The Microrchidia (MORC) family of chromatin-remodelling ATPases is pivotal in forming higher-order chromatin structures that suppress transcription. All MORCs share three features: an N-terminal gyrase, heat shock protein 90, histidine kinase and MutL (GHKL) ATPase domain, a central CW-type zinc finger (CW) domain, and a divergent C-terminal domain (CTD) with predicted coiled coils (CCs). MORC2 possesses multiple DNA-binding sites that undergo structural rearrangement upon DNA binding. Importantly, MORC2 mediates chromatin remodelling via ATP hydrolysis-dependent DNA compaction in vitro, regulated by the phosphorylation state of its CTD.

As a MORC2 neuropathic mutant S87L was shown to have residual ATP hydrolysis activity, we have identified and utilised ATP hydrolysis mutant S87A. We determined a 2.4 Å cryo-electron microscopy (cryoEM) structure of full-length MORC2 ATPase-dead mutant (MORC2S87A) in the presence of AMP-PNP. The AMP-PNP density was visible in the cryoEM map and at the same location as found in the crystal structures. The presence of AMP-PNP density near the ATP lid in MORC2S87A model, confirmed that this mutant can bind but not hydrolyse ATP, mimicking S87L variant where some residual ATPase activity is still detected. S87A mutant had similar DNA binding affinity as wild-type MORC2, indicating that ATP binding did not affect MORC2 DNA binding. The dimerised ATPase domain is well-resolved in all the cryoEM maps, but no density is seen for CTD to model in the full-length MORC2PD, MORC2PD-DNA and MORC2S87A maps. The lag time for DNA compaction by MORC2S87A was 3.5 times longer than that of MORC2WT, with an eightfold increase in compaction time. We found that MORC2WT compacted DNA into a large DNA cluster, whereas MORC2S87A, MORC2N39A, MORC21-603 and MORC2604-1032 variants did not. Our investigation of the MORC2 S87A mutant based on the patient variant S87L, which retains ATP binding but has significantly lower ATPase activity, showed significantly slower DNA compaction than MORC2WT.

>[2x]MAFTNYSSLNRAQLTFEYLHTNSTTHEFLFGALAELVDNARDADATRIDIYAERREDLRGGFMLCFLDDGAGMDPSDAASVIQFGKAAKRTPESTQIGQYGNGLKSGSMRIGKDFILFTKKEDTMTCLFLSRTFHEEEGIDEVIVPLPTWNARTREPVTDNVEKFAIETELIYKYSPFRTEEEVMTQFMKIPGDSGTLVIIFNLKLMDNGEPELDIISNPRDIQMAETSPEGTKPERRSFRAYAAVLYIDPRMRIFIHGHKVQTKRLSCCLYKPRMYKYTSSRFKTRAEQEVKKAEHVARIAEEKAREAESKARTLEVRLGGDLTRDSRVMLRQVQNRAITLRREADVKKRIKEAKQRALKEPKELNFVFGVNIEHRDLDGMFIYNCSRLIKMYEKVGPQLEGGMACGGVVGVVDVPYLVLEPTHNKQDFADAKEYRHLLRAMGEHLAQYWKDIAIAQRGIIKFWDEFGYLSANWNQPPSSELRYKRRRAMEIPTTIQCDLCLKWRTLPFQLSSVEKDYPDTWVCSMNPDPEQDRCEASEQKQKVPLGTFRKDMKTQEEKQKQLTEKIRQQQEKLEALQKTTPIRSQADLKKLPLEVTTRPSTEEPVRRPQRPRSPPLPAVIRNAPSRPPSLPTPRPASQPRKAPVISSTPKLPALAAREEASTSRLLQPPEAPRKPANTLVKTASRPAPLVQQLSPSLLPNSKSPREVPSPKVIKTPVVKKTESPIKLSPATPSRKRSVAVSDEEEVEEEAERRKERCKRGRFVVKEEKKDSNELSDSAGEEDSADLKRAQKDKGLHVEVRVNREWYTGRVTAVEVGKHVVRWKVKFDYVPTDTTPRDRWVEKGSEDVRLMKPPSPEHQSLDTQQEGGEEEVGPVAQQAIAVAEPSTSECLRIEPDTTALSTNHETIDLLVQILRNCLRYFLPPSFPISKKQLSAMNSDELISFPLKEYFKQYEVGLQNLCNSYQSRADSRAKASEESLRTSERKLRETEEKLQKLRTNIVALLQKVQEDIDINTDDELDAYIEDLITKGD>MEKFLVIAGMNAIESEELLLKVGEEIKRLSEKFKEVEFVFKSSFDKANRSSIHSFRGHGLEYGVKALRKVKEEFGLKITTDIHESWQAEPVAEVADIIQIPAFLCRQTDLLLAAAKTGRAVNVKKGQFLAPWDTKNVVEKLKFGGAKEIYLTERGTTFGYNNLVVDFRSLPIMKQWAKVIYDATHSVQLPGGLGDKSGGMREFIFPLIRAAVAVGCDGVFMETHPEPEKALSDAPTALPLSQLEG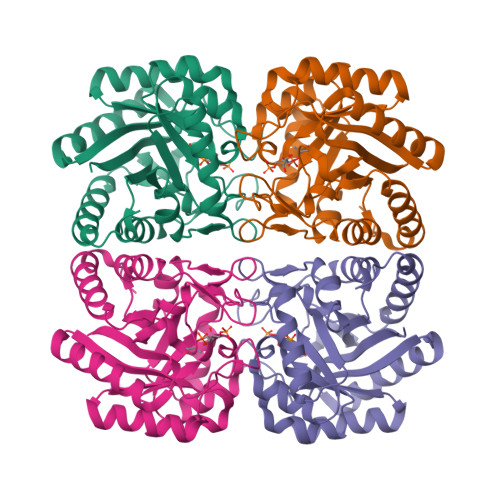IIEAILEIREVASKYYETIPVK[2x]(1~{R},3~{R})-5-[(2~{E})-2-[(1~{R},3~{a}~{S},7~{a}~{R})-1-[(2~{R},6~{S})-6-(4-hydroxyphenyl)-6-methoxy-hexan-2-yl]-7~{a}-methyl-2,3,3~{a},5,6,7-hexahydro-1~{H}-inden-4-ylidene]ethylidene]-2-methylidene-cyclohexane-1,3-diol 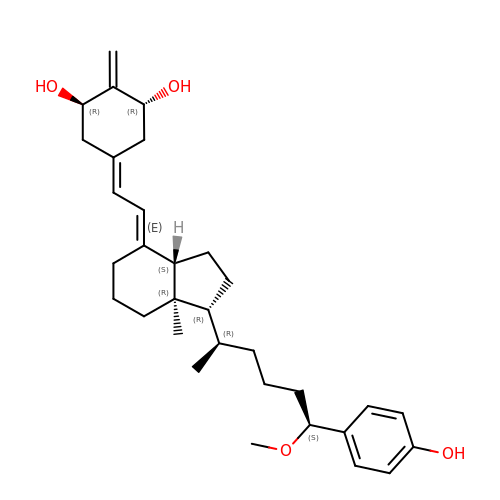| C32 H46 O4 | LNLTYAYGVNOEBQ-CLQLOTFESA-N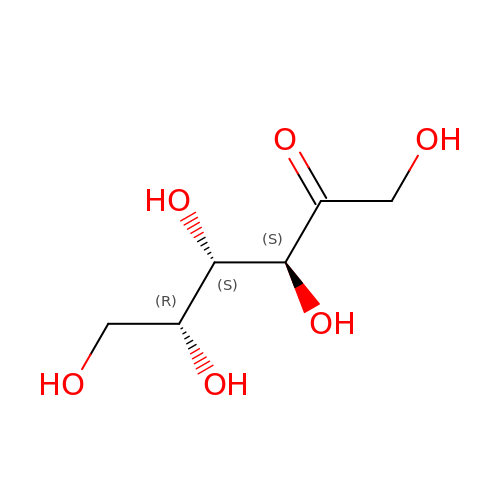D-tagatose | C6 H12 O6 | BJHIKXHVCXFQLS-PQLUHFTBSA-N N-[3-(2-{3-amino-6-[1-(1-methylpiperidin-4-yl)-1H-pyrazol-4-yl]pyrazin-2-yl}-1H-benzimidazol-1-yl)phenyl]propanamide 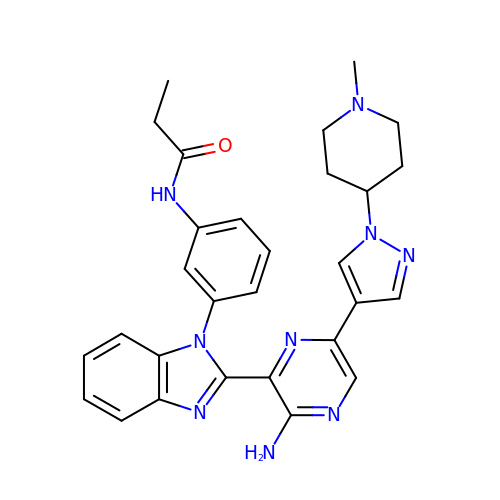| C29 H31 N9 O | KKUKNIKTWVWHBF-UHFFFAOYSA-N> QGTSSMADIGSLELFFRKKGESGEPLIILHGLYGSGDNWISIANELKDYFQVYLIDQRNHGRSPHADDMSYESMAEDLHEFIKSQNLESVNIIGHSMGGKTAMWFTAAHPDKVKKLIVADIAPGKYDTTSPNVKTHKKIIAALKSIDPSEAKTRKEIETQLSRYIDNVQLRM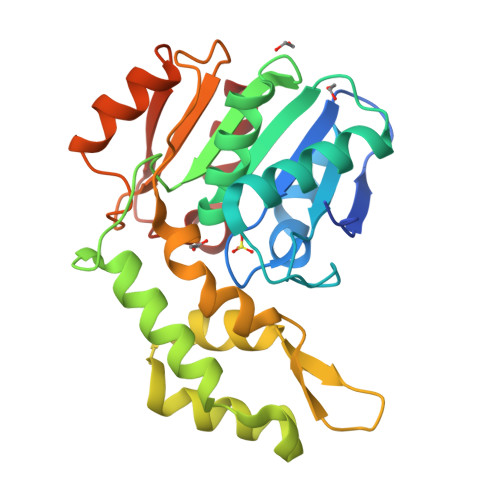FLLKNIERKEDGCYRWKINIDSIEKNIINIMSGITGIDIPVHVPALFLKGELSDYITDKDIPLIKEIFPDAKLVTIPGAGHWLHAQQPKIFIQKTLEFL De novo coiled coils (CCs) are particularly appealing modules for designing self-assembling systems as they are short, mutable, and sequence-to-structure relationships governing their folding and assembly are well established. For example, CC-Tri and CC-Tet exchanged with each other, as did the higher-order CCs, CC-Pent2, CC-Hex2, and CC-Hept. These two classes—i.e., CC-Tri plus CC-Tet, and CC-Pent2, CC-Hex2 plus CC-Hept—are structurally distinct: the trimer and tetramer have consolidated hydrophobic cores, whilst the others have central channels and are α-helical barrels. Similarly, peptides with Type II interfaces where the g, a, d, and e residues all engage in helix–helix interactions—namely the pentameric, hexameric, and heptameric α-helical barrels, CC-Pent2, CC-Hex2 and CC-Hept—also exchange with each other. To address this, using the insight from the data and analysis presented here, we have tested two different strategies for increasing specificity of coiled coils: (i) alternate placement of salt bridge-promoting residues, lysine and glutamate to discriminate the tetramer from the trimer; and (ii) incorporation of hendecad repeats to separate the α-helical barrels.

Variations of this 3-4 spacing can lead to alternative CC sequences and structures. For instance, in 11-amino acid, hendecad repeats core-forming residues are spaced 3-4-4 apart at the a, d, and h sites of a → k repeats (Fig. S38†).16,63–67 Consequently, while heptad repeats drive association of left-handed CCs, hendecads lead to right-handed quaternary structures (Fig. S38†).16,63–67 We reasoned that replacing heptad with hendecad repeats at different locations in the pentamer, hexamer, and heptamer sequences should alter the hydrophobic seams and, in turn, might confer homo-specificity in the resulting sequences. For CC-Pent2 and CC-Hept, initially, we replaced the third and second heptads, respectively, with hendecad repeats to give CC-Pent2-hen3 and CC-Hept-hen2, and using the Leu-at-h variants for both. Unfortunately, FAM-CC-Hept-hen2 was not soluble in PBS buffer, so we switched to a heptamer sequence with Ile in the a sites and Val at d and h (CC-Hept-IV-hen2). This proved more soluble and retained orthogonality. However, overall, this revised set of peptides showed significant improvements in orthogonality across the whole set compared with the original basis set going into this study. The second strategy differentiates the α-helical barrels, CC-Pent2, CC-Hex2, and CC-Hept, by introducing hendecad repeats in a pentamer and heptamer to give CC-Pent2-hen3 and CC-Hept-IV-hen2. Fluorescence measurements show minimal exchange between a revised set of CC peptides: CC-Di, CC-Tri, CC-Tet*, CC-Pent2-hen3, CC-Hex2, and CC-Hept-IV-hen2. We have denoted this group of peptides as the Orthogonal Coiled-coil basis set.

>[7x]XGEVAQAIKEVAKAVAAAIKEVAWAIKEVAQAIKGX> GSHMASPNGQTKPLPALKLALEYIVPCMNKHGICVVDDFLGKETGQQIGDEVRALHDTGKFTDGQLVSQKSDSSKD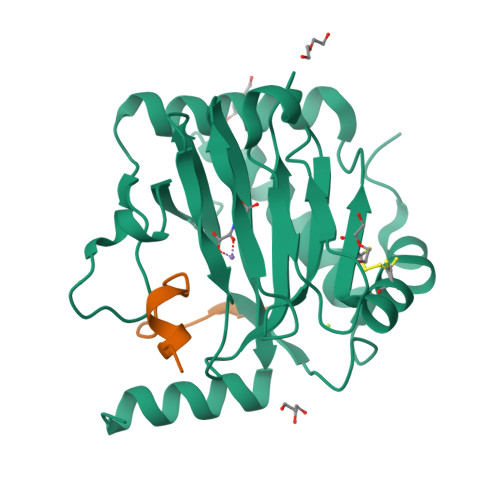IRGDKITWIEGKEPGCETIGLLMSSMDDLIRHCNGKLGSYKINGRTKAMVACYPGNGTGYVRHVDNPNGDGRCVTCIYYLNKDWDAKVSGGILRIFPEGKAQFADIEPKFDRLLFFWSDRRNPHEVQPAYATRYAITVWYFDADERARAKVKYLTGE;> ELDLETLAPYIPMDGEDFQL> ASSRVIVHVDLDCFYAQVEMISNPELKDKPLGVQQKYLVVTCNYEARKLGVKKLMNVRDAKEKCPQLVLVNGEDLTRYREMSYKVTELLEEFSPVVERLGFDENFVDLTEMVEKRLQQLQSDELSAVTVSGHVYNNQSINLLDVLHIRLLVGSQIAAEMREAMYNQLGLTGCAGVASNKLLAKLVSGVFKPNQQTVLLPESCQHLIHSLNHIKEIPGIGYKTAKCLEALGINSVRD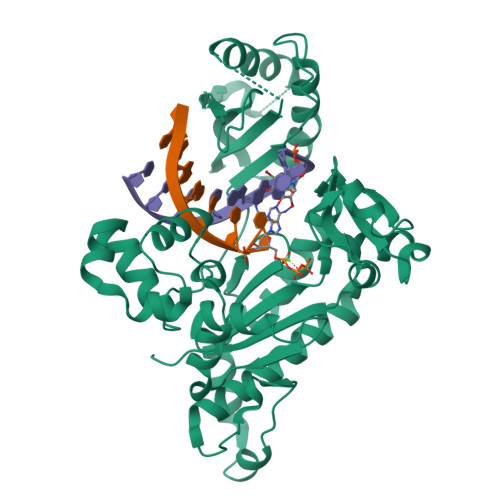LQTFSPKILEKELGISVAQRIQKLSFGEDNSPVILSGPPQSFSEEDSFKKCSSEVEAKNKIEELLASLLNRVCQDGRKPHTVRLIIRRYSSEKHYGRESRQCPIPSHVIQKLGTGNYDVMTPMVDILMKLFRNMVNVKMPFHLTLLSVCFCNLK>[3x]GSHMSEPTSSSSLDITSNCIIETPLQPSDFLPKSANLFPKFPERISVDSWELWEFDTFDTNGSVAFGCSLYRDARGVEQGGFHAEVNALWPDGTHWGETLYFAVSEVVENSDGTTGGKWLSKDGGSITFHIASDYTAAALDFNVPGKVSGTMELRNHANVSPTSNLPASDAEAQLCPGVYYTFPMGPVATSVTATFSSVGANGESRELFISSGYGGMVRGWSARPWPTFM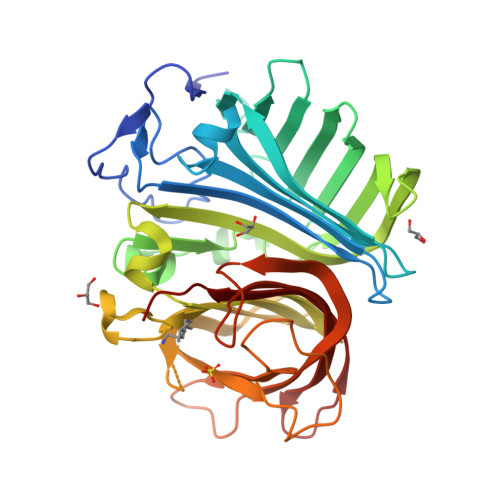NDAYYVVAQVGPYMLQILRTLGSVFVQHKPFAVARLYLDGSLVSAANTVVGDELTAHADDVKGDAVRLTKVQPDEKSQGLSGKFRDGNVGYVLEFAKKDSEHGWTFQISHKRAVWSEPTSAPGPDGTGKSGWIEAISGGAKGENYEGHGFGGQLQIPVP>GAMGSMSKQFVRSAKNLVKGYSSTQVLVRNATSNDNHQVSKDSLIELAEKSYDSADFFEIMDMLDKRLNDKGKYWRHIAKALTVIDYLIRFGSENCVLWCRENLYIIKTLKEFRHEDDEGIDQGQIVRVKAKELTALLSDDERLNEERNMNIKGRNRKGRRR[8x];>[8x]GAMGSMSRIDSDLQKALKKACSVEETAPKRKHVRACIVYTWDHQSSKAVFTTLKTLPLANDEVQLFKMLIVLHKIIQEGHPSALAEAIRDRDWIRSLGRVHSGGSSYSKLIREYVRYLVLKLDFHAHHRGFNNGTFEYEEY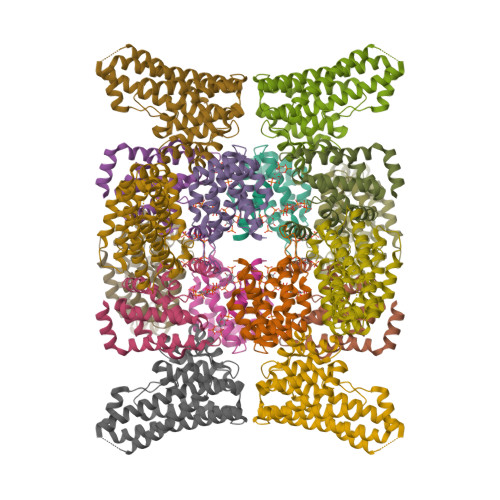VSLVSVSDPDEGYETILDLMSLQDSLDEFSQIIFASIQSERRNTECKISALIPLIAESYGIYKFITSMLRAMHRQLNDAEGDAALQPLKERYELQHARLFEFYADCSSVKYLTTLVTIPKLPVDAPDVFLINDVDESKEIKFKKREPSVT> ICQFKLVLLGESAVGKSSLVLRFVKGQFHEYQESTIGAAFLTQTVCLDDTTVKFEIWDTAGQERYHSLAPMYYRGAQAAIVVYDITNTDTFARAKNWVKELQRQASPNIVIA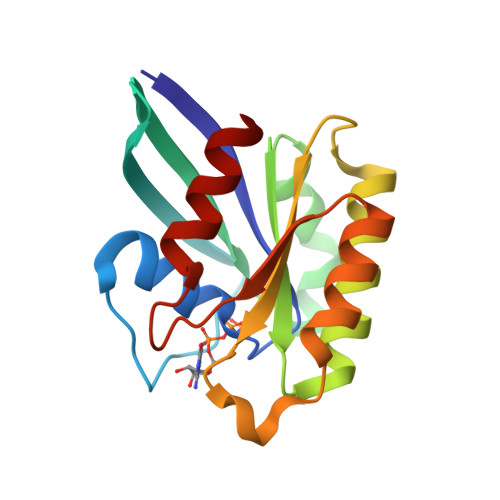LAGNKADLASKRAVEFQEAQAYADDNSLLFMETSAKTAMNVNEIFMAIAKKL> GSHMPTTAASTPDAVDKYLETPGDENEHAHFQKAKERLEAKHRERMSQVMREWEEAERQAKNLPKADKKAVIQHFQEKVESLEQEAANERQQLVETHMARVEAMLNDRRRLALENYITALQAVPPRPRHVFN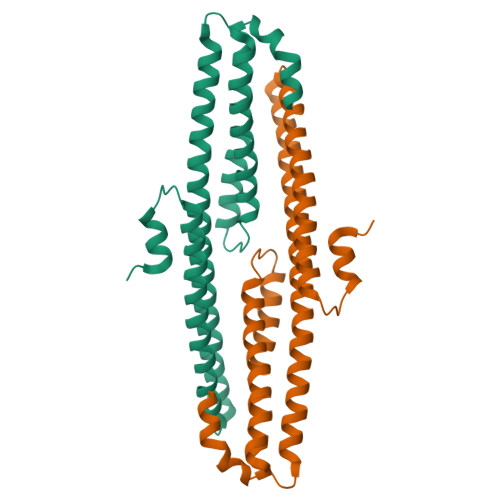MLKKYVRAEQKDRQHTLKHFEHVRMVDPKKAAQIRSQVMTHLRVIYERMNQSLSLLYNVPAVAEEIQDEVDELLQKEQ> AIAGAAGAUCUUCUCU

A long-standing challenge in primordial nonenzymatic RNA copying chemistry is the biased incorporation of C and G over A and U due to differences in base pair strength. We hypothesized that 2-thiopyrimidine substitution could help overcome this bias since A:s2 U is a stronger version of the A:U base pair, and I:s2 C is a weaker version of the G:C base pair. This study explores the efficacy of a potentially primordial genetic alphabet consisting of s2 U, s2 C, A, and I. Our results show that A:s2 U and I:s2 C pairs are isoenergetic and isomorphic. All seven oligonucleotides crystallized within 2 to 3 d at 20 °C under their optimal crystallization conditions, and we solved their structures by X-ray diffraction at resolutions ranging from 1.3 to 1.6 Å.

The closely related sequence ICS1, 5′-AIA GAA GAU CUU CUs2C U-3′ (24), can form two I:s2C base pairs in the same positions. The I:s2C base pairs in the ICS1 and ICS2 sequences exhibit only two hydrogen bonds between O6–N4 and N1–N3, due to the lack of a 2-amino group on inosine. These two hydrogen bonds are located at the same position and have similar bond lengths as in the A:s2U base pair. The superimposed I:s2C and A:s2U pairs show that these two base pairs are isomorphic. The missing hydrogen bond is presumably the main reason that the I:s2C pair is weaker than the Watson–Crick G:C pair. However, the hydrogen bond between N1 on I and N3 on s2C has a slightly shorter length (2.7 Å) than both Watson–Crick G:C pair (2.9 Å) and G:s2C pair (3.0 Å). This stronger hydrogen bond may partially compensate for the loss of enthalpy due to the missing third hydrogen bond. In contrast, the absence of the 2-amino group on inosine and lack of an N2–S2 hydrogen bond results in the I:s2C base pair exhibiting no significant changes in the base pair opening angle, thereby making it possible to enhance the N1–N3 hydrogen bond. The distances between C2 on I or A and S2 on s2C or s2U in all structures containing I:s2C or A:s2U base pairs are consistently 3.5 to 3.6 Å, falling within the typical range for a C–H⋯S hydrogen bond. This suggests that a third hydrogen bond may form in both the I:s2C and A:s2U base pairs, but not in the I:C or A:U pairs.>[4x]SNAMNPIEFWFDFSSGYAFFAAQRIEALAAELGRTVLWRPYMLGAAFSVTGARGLSSTPLKRDYAQRDWARIARQRGLTFRPPADHPHVALAATRAFYWIEA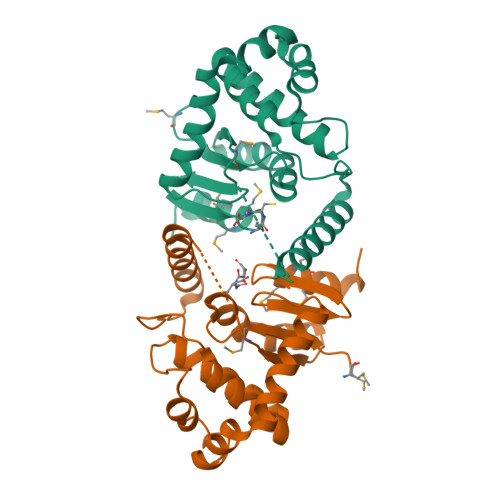QSPDAATAFAQRVFDLYFSDRLDTASPEAVSRLGPEVGLEPEALLAGIADPALKETVRKIGEDAVARGIFGSPFFLVDDEPFWGWDRMEMMAEWIRTGGW>[2x]HNTT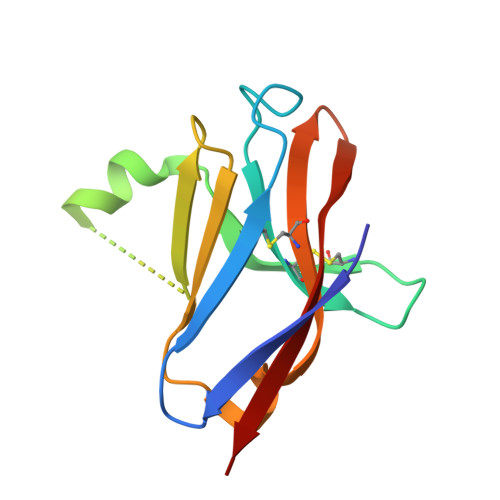VFQGVAGQSLQVSCPYDSMKHWGRHKAWCRQLGEKGPCQRVVSTHNLWLLSFLRRWNGSTAITDDTLGGTLTITLRNLQPHDAGLYQCQSLHGSEADTLRKVLVEVLA> MTDNAPQLALRDVAARQLANATKTVPQLRTITPRWLVRLLHWTPVEAGIYRVNQVKDASQITVACSERDESELPETFVDYIDNPREYLLSAVNTVVDVHTRISDLYSNPHDQIREQLRLTIEIMKERQESELINSREYGLLNNVAPGQLVHTRNGAPTPDDLDELLIRVWKEPAFFLAHPQAIAAFGRECTRRGVPPATVSLFGSSFITWRGVPLIPSDKVPLENGKTKILLLRVGESRQGVVGLYQPNLPGEQGMGLSVRF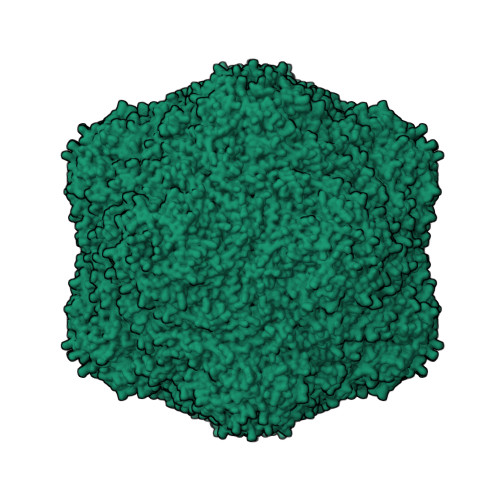MGINRKALASYLVSLYCSLAVLTDDALAVLDNVDVTQYHTYRYNSGHHHHHH>[4x]NLFSKDIFKFKLVDQFFPFYYKNNKGEYEGLIFSILDKWAKDNNADIMVEHIDNLNESEIEDEAIYLGLTYNVKLNDFFYFKSELAR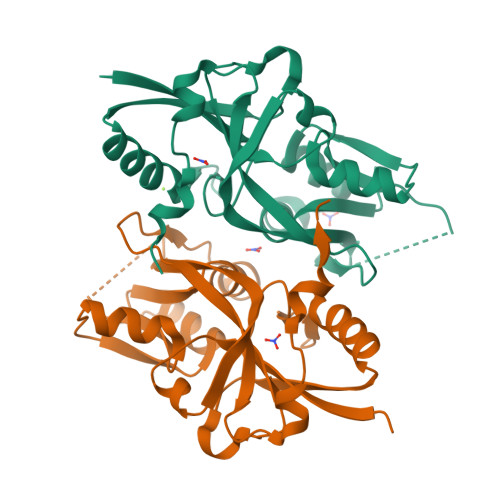SISILFFKNSNKKYKNTHSTFLSNFNIGVIKNTIYEDILRLKNVNTIFLADNSQELVLALKNDKVDYIYGDCKTLHYIANNFLSEDLVIFTGDVFYSIKNRVAISRNAPEIVKNLNLDLFSYLMKMPEELVFSFLDSNAK> MEKLDKIRMSQKLS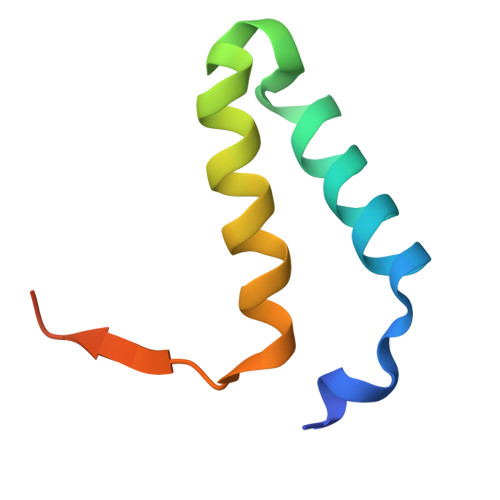CWQHILTTLGTSSKTEQEWNTFFKGFLESWRKPYCIQTSCDPSIPL> MASMTGGQQMGRDPNSSSM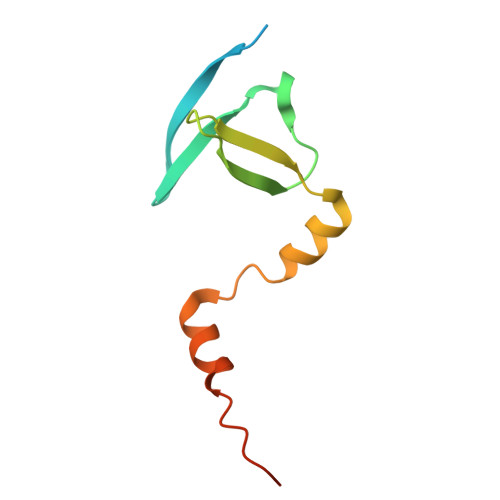LTKVFQSGNSQAVRIPMDFRFDVDTVEIFRKENGDVVLRPVSKKTDDFLALFEGFDETFIQALEARDDLPPQERENL>GPMRTTLTGTASVLDTTLTRLIDDVIENGSSFLADDENLQHYKQHLSHLETASKIALLRECLCVRPPLPLLPEDLLQNVDSILTRVRQHKILTPIFSLSPSRLIKHGDLGATRIHLWRGDITTLTGVTAITNAANSQGLGCFQPTHRCIDNIIHAEAGPRLREECFQRMQARGKELEPGEVLVTEGHALFASSVMHTVGPQLKRGASPTETERRQLAKCYESILEALELLPSDEDGSKSIALCCISTGLFAFPADEAAEIAVSTVTSWLQKHPSTTITDVIFNTFTQSDTEFYSKLLGPSHTKSISPVENTPQGSLSLAREWLSSADAVLVTAGAGLSAAEGLDYHSRDLFKRNFPGCLKFGLTSLYSVFGFNDWPSEEHRWGYFFTHLNMVANWSNTPTYQTLIPWLRNFGQDAFVRTSAADGLFLANGWPKEQLSTPQGSYGYLQCLNNCRVDAVVPSAPLVADAMPHIDKATQKLMDPSKIPLCRFCGSKMSICVRAGSWFNQAPYQEGEAQWKAWKSRVLREKKNLVILELGVGMNTPGVLRWPNEDLVMRSDGRVKLIRVGMGPEAMVPWEQEDEGLSTCVQGDIGRAIPLLLE[2x]

In some pathogenic microbes, the response to oxidative stress is controlled by a SirTM/zinc-containing macrodomain (Zn-Macro) pair responsible for establishment and removal of the modification, respectively. Strikingly, however, the “catalytic loop” found in all other MacroD-type enzymes (also termed “loop 1”) is replaced with and extended loop containing the zinc-coordinating Cx(4)HxC motif, here termed the Zn-loop. To gain a closer understanding of the functional role of the 3α-bundle and coordinated Zn2+ ion, we solved structures from the three sub-branches of Zn-Macros namely from S. aureus (SauMacro), Methanobrevibacter oralis (MorMacro), and macrodomain-fused SirTM protein (Mfs1) from Fusarium oxysporum f.sp. cubense race 1 (Foc1Mfs1) in their apo form as well as of S. pyogenes (SpyMacro) and MorMacro bound to ADP-ribose (ADPr). In all structures, the Zn2+ ion is tetrahedrally coordinated with three metal-coordination residues within the Zn-loop, while the fourth coordination-contact is exchangeable and is provided by either ADPr, a water molecule, or a symmetry-related protomer within the crystal.

In the Foc1Mfs1 structure, the Zn2+ ion is absent from the macrodomain, while the structural Zn2+ ion coordinated within the small subdomain of the SirTM domain is still present. This absence leads to increased flexibility and distortion of the Zn-loop within the crystal structure as indicated by the loss of density information for the region (residues Asn133 to Ile147). The Zn-loop appears to be partially stabilized by contacts with the 3α-bundle. In particular, the contacts made by Asn46 seem to contribute to the overall stability of the Zn-loop and the exchange of this residue to cysteine (Cys61 in Foc1Mfs1) within the Mfs1 branch may contribute for the absence of the Zn2+ ion from the Foc1Mfs1 macrodomain structure. We therefore created macrodomain only construct (Foc1MOD; aa 1–305) and compared its zinc-binding ability to SauMacro. In line with our structural observation, the amount of zinc copurified with the WT Foc1MOD protein was reduced by approx. 75% relative to SauMacro. Surprisingly, neither MorMacro, which arises from a minimal operon containing only the Zn-Macro/SirTM pair, nor Zn-Macros derived from Msf1 fusion proteins could demodify SpyGcvH-L. In contrast, all Zn-Macros could demodify Glu-/Asp-ADP-ribosylated PARP1 E988Q. Identifying the physiological substrates for example, for the Mfs1 fusion protein would not only elucidate their substrate specificity in terms of attachment residue and sequential context but also reveal how these proteins contribute to the oxidative stress response of pathogenic fungi.> NLYQFKNMIQCTVPSRSWADFADYGCYCGKGGSGTPVDD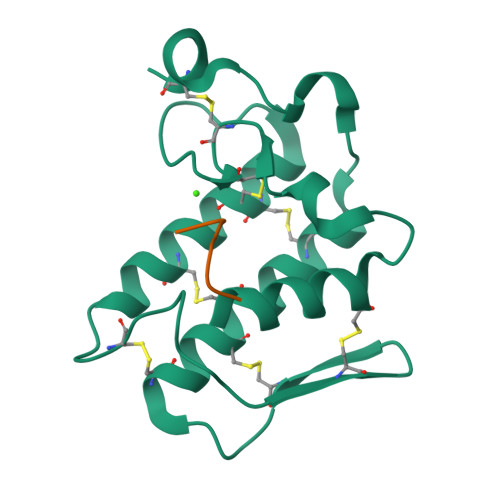LDRCCQTHDNCYNEAENISGCRPYFKTYSYECTQGTLTCKGDNNACAASVCDCDRLAAICFAGAPYNDANYNIDLKARCN;> KGAIIGLM> Q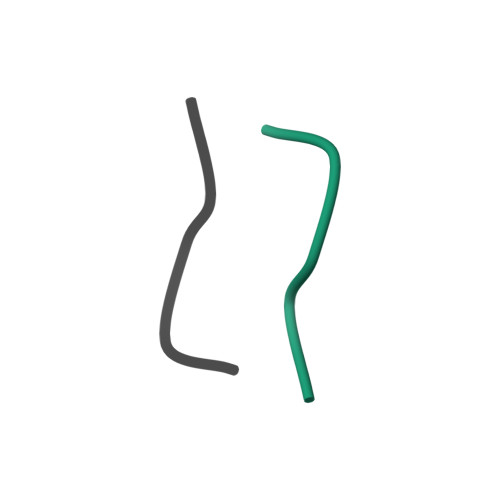TRPDQTRPD> TCGTCT;> GAACGACACAGACGACGA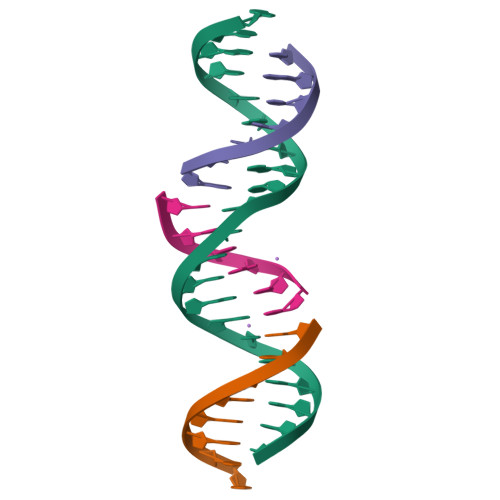CTC;> TCGAGTCG;> GTGTCGT>[2x]MQALRRGAAIPSRLLPRRDSWMSLAPFVAPNNAAAWRKLRDGAQEVQTVIERQSTPGKPQQIDWAKWESQIAHKDILNCLKTFYTNQVQILDRALGALETAKTPAPCEGAEKGWALFDAALSACAKSVEKSEELLSNGARALWVSCSNPPVWKVNTNEWLDSDQYWQAFVEKHHFYSQYQPGVVDPEAPQEVEAFKQAWHSRMGKFNDRSDTPMLYAYMNELPSWEYYDLHRSAFLEHMTYFLVRTGGDFRFFPEMPPWQWLAHMENLRFKLLSVAQSRRSQLQLANLERERALDFLPVDVEHHGEEYTQKFLQYETELFQACAARLMGHFMFLCDPFIPVQSAEALSAVTRVDNGKGKLFSLGDDVNALFYLPEQQRRDVERPTQAVQTLLGHLEATGRPFNPCYSELLHVHAEVLEERGEHWLTAPGECVSQAFLRRLRTDDPAYEVYCSYFKEMYERFAGAKEVSMEDGRKRLATIEKNAQEEAAAYGLALKTMGSAELAHKAREGAAKLEQLRKAQEKAAGKSAQTVQENKM;>[2x]MNFSSSARWLAVRQSQTLGHTTRATVAAGRRVLAHSPAATEFTSFQSLHIGGDVCKLPLAVALGAAPSALGYGSAKHNQQRQYATLGSGWSFSKVQYTKYRITKPWTTDTTFDDIILSQPSKEDFAKFTKEAPLFLRFLKLVTDVEGRQEAFIQFAKRCENGLTVEKDVYVTKKELVDCLWKNGYTDTEINAFEIAFPADYKFHYPELAVLFDLTEEDCYKYCIRQRAATPEELVELKYTKPKNLVSSYGLCFLGVWFGLSNTVLSNAWFYSKTFPFGAVFYMLGSYFYRDIREKLWKEEKSLIHTAQENKNMGEESVYKQMKKYATDTKCLDYLSTFRTEVEDQIANYKVALVSQMRRQLTERLVEKLNGIQQAEKLIQGSLQDVMIREIVSSFKDLYKSRPELHDAAMQSAIQGLSGSDGAMDPVGAHFKASLQELAKVNLSTATADPMGTVVQRVAAVFQKREKEFLDTFTVKATEAQEIKTIVDKCHKGNTFDFHALSDEELRRLEQLYSTVNNRVGFETIHENSIKPVAPLSENSKGFVEFVNTQLEITKAKLRNARLTAFAHAFV;>MGGGGGGALNKLFPGYKDKIWMKVPVQWRQQMIQHWNKSYEKQVYSESVALNRTFQARNQLVLDRLKPSGAYRLPAVDYKRQLSRGTLVEGADFYLPTAQEQQRLARHFEPYSEQEQEERRKFRFQSISVYLAVALGASFVHDYFYQRRPVAWCLEKEPPHPPSYPFWFKSLFHSHDIPSVRRGYEVYRKVCATCHSMEQLHFRHLVGEV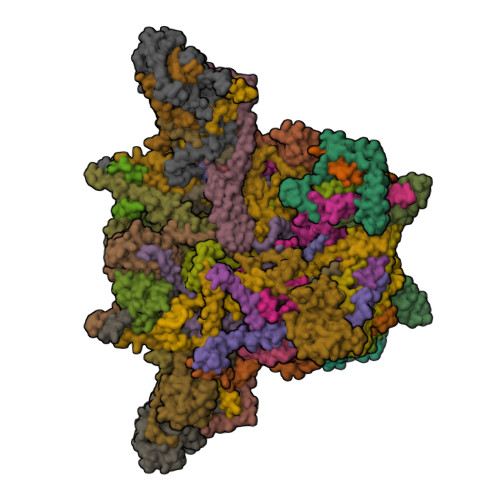LPEKRVKQIAAEYDVTDGPNDQGEMYTRPGILGDAFPSPYPNEEAARYANGGAYPPDLSLITAARHFGPDYLMALLGGYRDPPEGVELRPGLYWNVWFPGNAIAMPPPLMDEMIDYEDGTPCNISQMSKDVVNFLTWATEPTADERKLYGLKCVSAIAIGTVLMTLWWRFYWAMYATRRIDFGKLKYL[2x];>MSPVGRLFLGSKLPAQTWQSFRLQPALPQFAQKRFFSGGAAKPSWHVAREHRFGPTLPDHAYYGEHATYNYFVLFIRGMRPYLEKIFGDCASTIKNAAVAVYRPVNAFVVKHNPDLRLQFVAFASFIATHMAITKEFNDMYQRLVDITSLLELQAAQLHASEGFWDSESEQQEARLQRHAEHRNDLETTWEEALREATLARNFDVLVSYLNHGTSDGCGEHGACGHSGQNGIPPSVTWNFNAMPYGKENPDTKTFPIPDHEQPYRAFSLGFTANNLSGNWGDYIDRQDNKNALMRPARMMFTDVFIPTTK[2x];>[2x]MGEKQEEEGEEEKEGKGEGGGEGGREEEDEDGSAPVVSWLRIVEERECHEETDEAPETKIALPFSAQRSSRGFEARQVEVLVSANSAFLLSVLLASLFLSSSLPSFCPPRFLLSVLLALFKDKMAGDAPAAAAAPQQAGRTASASGVRTPGYLDLVGHSLKATSMDHGMQYSSIYWETSHRTYLPFWASLTQKFSWKIMDDQIRSFLRLPKPVTTEPFVFSSGSPYIRRYFGDADISVPVPLHAPAHFAFVPTGTVSPWEETGMETGPQGAAARGAAATAFRAVLESAWKCDIDEQIKEKLHSRAGAGAFHASGSTGGCPIPTDF;>MALNRVPSRVLPFAVSGVYVHPRNACRLPAAAAVSSVPSSVSAFSSRTNFLSRSSSAVMSHPCAATARHFSFAIPPANAAALADPLPATPTPPPVFEAVSSASSGIASGTNALKNVEEVSTMERYEAAVYEESFKKPIVCLFFARFSLQSKVLLQPFLDFAASASNNATFFLIDCDRVPRAAYHARVENVPSLVVMKGDDAFRQTITDSVGVKTAGDLIQEARSALDQVLRLDQQEGGTKLQPGVSSYTHHIGVDNLNVYRKGWPVA[2x];>MQNGVFTRENADFLVKSGADSPSSQSLLLRTSPSPLSLPRRRFIFLRSASVDLSERSSLACLAPFFCLASGVCLRSAFSLPFFARRGRPCLFFIFIFFFRVSFTANFRGKRVKMAASTIPISQWPSLLYAPPSSPANPAVEALPEMQFDDLHYPRQMLLCRGAGYSLEQCNRMAQPDARVTPENPAEKLLKEEAVAAIACLSQREGGKDEQCRYYIERMYKLANKEKQPEPGTLSKASTLACKLLGIHRPEA[2x];>[2x]MAETREGGQSGAASILGAEAFPELLSKVPLNPQMDEDKHFNKYKWGNEPIPVNRRTGSRMNSSIYDNRNHEAVRHPWSTDARTFHPNDNPEADRINTQYSNMVSDSFPEGGFSDAPRFSSNWERLLAYHHGLYSPEKFNSTTKTADEIRLAVNDFAAKVHADDPKNACKYLMIEEFKCLQSAQARIDPQGAATKCVKWFNEWRQCAWDQEKMVKGYNYIEDRRARKHKPYIGAPDLQYS;>[2x]MPSSSSEDAQGGNRFECVSNSTSPRRKNATKDEAACLQPRRSAVSGPREDVLCIRTTPQPHVRRGKSGPGRRKRMRFGRERERRDKKRGEGERKRTRFPFLRLHIEGGNANSRRPLCFPSRHSLLRNHYGSLSMAFRKVSPPKAPMSVFEARSSFLDLEQCARAAGPQRWEAECQGVRQRALQAAADVMSRECGAYGDSFFQCYRHGFRLEACQGEKATMQLLRCQRMVADRLVPL;>[2x]MGLSPAFAATAGCRLASPVANSSRFLSLLRLSRPRLNAAAPAAEAAKTLERNVPMKEILQPLWVVEPPNFLRQPVWKQFWEAQFANRSFFFFGNAWTSAAAFAFFIWWSRVFDPPPKERLDRYWLNSPKFRILSAFHNPGKRPGLKISLMTYEARYCYRGLDHPFTLNEMKDFLFKLREQYLVNKYEGIQFPFVFRQFNRVSTPGTLEVHTSPALQQQPHFHEEAAGHH;>MAAGSRFPFCTAARLSSRGTLPRLGEATFFAGAESQRSAGAFAKTLQRPFLRAPSTQLFPVGNRLGVSSARALVANAMEPRRFFAAAASAKATHALQPTGTGSVAFTRPGQGSNAQFQTSLADKTRGLLGVGFLRPTKMASFAATFLLNFRFYFMYMARTTFQAVRPLLAFSVFGEVMKLVLATMSSGLFSFLFSFVLAFEVFYFFLQCYISYTFLTMFFTVLF[2x];>[2x]MTALPPPPSANVAVSFTAAPAEPLSRGEVKAASLKLELQNIERELKDWWMSRKILRDRNIGLFNLLQHHNFAGLSVNNAKLSDSQRVMWTDLVQGKPDVEDKLSVDAREMKVDMYEKLFKQAADLENPCRMPGVAYLRCLRDTLTETQSARRSSCLNAFSSFDACRTGLLKQQSAAVENSLVRQNMADVRAKALFERRAVLLDLVEGK;>[2x]MNTFFLTPAAAAARRVAVSFFARSSASGFPQHRVALRPFPSQRPAERAHNLAKSQTLRSVKAHGRQSGKKEQSTESGGRRGFRAAVGAGTGCMLAASPMLFTDYDNTASPKSELIFMAGNALGYCTERFFENEYGQSIFMFALGLAYLAMLGHEGKIHGAVWRMKHLFATNFKMVGHPRYAYALPKNPLLQDAAPTKTGSTSAKK;>[2x]MSGDSVAPHQRAACEQLHSEYKQCLAKNGRTHFSACTDFHSKLRACENMLGTSYCIDEGINLMKCTKNPDPSFCAKEFVAMRECNRPQGPHLVLSSSPSSPPHYELRPEVKHLYNVDSTDLGSAVAPVRSKEQLDRVADSLKADLNLPGYGHIPYKWESLRPNPGA;>MAFAGAAAPLGVKGRSVFAGMRSFIGQRLGRLYDSFYYSQSSTKYVMVFLFPAGIFYTRFRADTKLGYHVFINEEKLYPDYSQNYFDTKWTNGRKVYLDDETTVEQLKAQIYGGKAAPENVKVACRGRVFEDADNVAMAVRAFCKRDPRLLLFQDNL[2x];>MSPPTASASVASSGSSPHMDRLLGDLKLLAAYDSAAGWQEPKAMESAFQSLSWDDADVLKALPQYLNCRGEQKRRVDFAYAALCPRPVDEKDPKQTLMSLWMKARLFSYDQKHPFVLSPFAATDKSTSAGAMTAEKPF[2x];>MVRNQRYPASPVQEIFLPEPVPFVQFDQTAPSPNSPPAPLPSPSLSQCEEQKDRYRDISSMFHRGVAGAEQVREAYNSMAKCFRRVSVAEVLESDPAFRQARNFTMDLKQAEDDQRYKQLQYGRVPSILTKYHL[2x];>[2x]MLNFIPKRCPSVSLLFGKRPVQRIEVGQARHQLEIPVETIEKIYEGVDSRLEYHNKDYNAMKWKDFMKLKLDAYHLLEASQSETAAKSALSDLNWFSDLADIYSGQQTMAEMDVALKAQGEQKLSYPIQGKNIK;>[2x]MSWATRLLRMSSPRLGLLPLGRSVKLGGAKERVSFSQFFDSEYFWTKANVGPFFLFLFTSPFWYQGIKTVYASCRYRKLNEREIISDRYTWLHERMLEDEVERVLLEQVPAGGFDKTRPGLLLGPSTL;>MPAPAASGAAAVLSKDIARSFRWMQAFAAVKGKPTAGSCAAGTAVVNPEDPTKVTLKGRYTNFSLQHIWEKYDYLQTHLLLRECMLSQVAKNPRLLDPEINAGLTPTVFMRVPPETQDPETQAKAAPQKGQAN[2x];>MATPPLQDGAPTNGGAATKPSCGARLQNFARMAIKGPSVPHSILFGVGAGCCAYAGYYLYRAMRLTFFDTESVALQSRLRYAEKQKLFHQELDRELAAGHIASLVAEYDPVATRLPFQPMQDRYRV[2x];>[2x]MGFHFQQYIAMAGRAINPVQWTRAWRRMEGKSATEVYRDALAWTNNQFAQISRASQYRAWWWQNPLGMGLVLYGTYKAWHMIYMVRKQKKTAQLVAAAYGQGGQWLNPVPR;>MPFMWRQRAYCAPVPSAFASQQPNGLGGEAGVRKPLLRSNSESLSVFSQIPDGLLGHTTSVTMGNSDIFFLPKPSNLLKIALPAFVFMPNLTIFTRAFPFYAHTSA[2x];>MSTSPGLAFANLTLLLDVPQLPAIWAVNAWRELNGLFTEMKTLAGTSDLLYPSNRYNPQNEKTNRMGRPRKYNHGEWMFGNSY[2x]> MGSLSREDMESVLDKMRDHLIAKNVAADIAVQLCESVANKLEGKVMGTFSTVTSTVKQALQESLVQILQPQRRVDMLRDIMDAQRR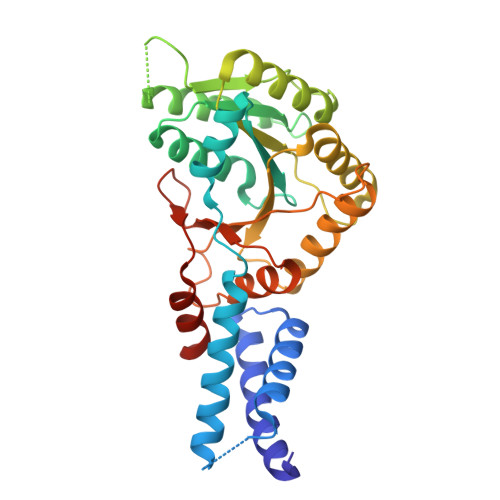QRPYVVTFCGVNGVGKSTNLAKISFWLLENGFSVLIAACDTFRAGAVEQLRTHTRRLSALHPPEKHGGRTMVQLFEKGYGKDAAGIAMEAIAFARNQGFDVVLVDTAGRMQDNAPLMTALAKLITVNTPDLVLFVGEALVGNEAVDQLVKFNRALADHSMAQTPRLIDGIVLTKFDTIDDKVGAAISMTYITSKPIVFVGTGQTYCDLRSLNAKAVVAALMKAHHHHHH>[6x]M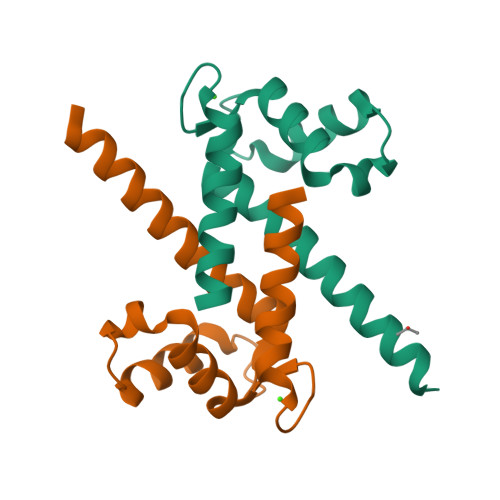PSKLEGAMDALITVFHNYSGSEGDKYKLSKGELKELLNAELTDFLMSQKDPMLVEKIMNDLDSNKDNEVDFNEFVVLVAALTVACNDFFQEQQKKRSK> CRFETSELQASVMISTPLFTDSWSSCNTANCNGSIKIHDIAGITYVAIPAVSMIQLGNLVGLPVTGDVLFPGLSSDEPLPMVDAAILKLFLQLKIKEGLELELLGKKLVVITGHSTGGALAAFTALWLLSQSSPPSFRVFCITFGSPLLGNQSLSTSISRSRLAHNFCHVVSIHDLVPRSSNEQFWPFGTYLFCSDKGGVCLDNAGSVRLMFNILNTTATQNTEEHQRYGHYVFTLSHMFLKSRSFLGGSIPDNSYQAGVALAVEALGFSNDDTSGVLVKECIETATRIVRAPILRSAELANELASVLPARLEIQWYKDRCDASEEQLGYYDFFKRYSLKRDFKVNMSRIRLAKFWDTVIKMVETNELPFDFHLGKKWIYASQFYQLLAEPLDIANFYKNRDIKTGGHYLEGNRPKRYEVIDKWQKGVKVPEECVRSRYASTTQDTCFWAKL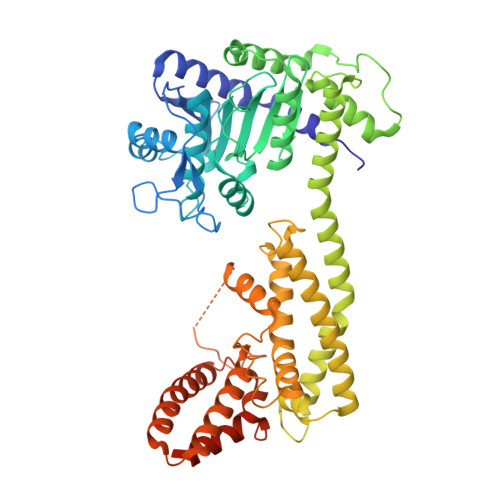EQAKEWLDEARKESSDPQRRSLLREKIVPFESYANTLVTKKEVSLDVKAKNSSYSVWEANLKEFKCKMGYENEIEMVVDESDAMET> DPKRLYCKNGGFFLRIHPDGRVDGVREKSDPHIKLQLQAEERGVVSIKGVCANRYLAMKEDGRLLASKCVTDECFFFERLESNNYNTYRSRKYTSWYVALKRTGQYKLGSK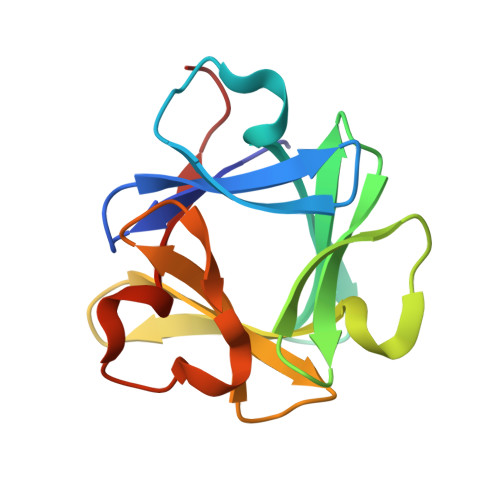TGPGQKAILFLPMSAKS> MSLRLGDIAPDFEQDSSEGRIRLHEWLGDSWGVLFSHPADFTPVCTTELGFTAKLKDQFAQRGVKVLALSVDPVDSHLKWIDDINETQDTRVNFPIIADADRKVSELYDLIHPNANDTLTVRSLFII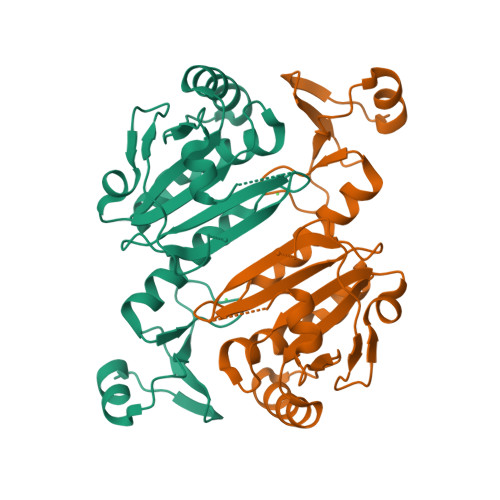DPNKKVRLIITYPASTGRNFNEILRVIDSLQLTDEHKVATPANWEDGDEVVIVPSLKDEEEIKRRFPKGYRAVKPYLRLTPQPNR>[2x]MQWSGARALEALLTVAGELRGP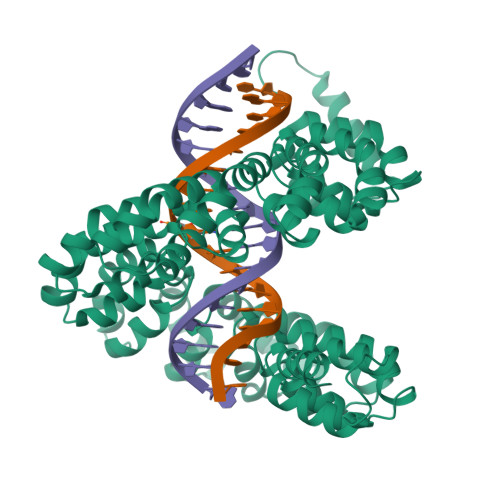PLQLDTGQLLKIAKRGGVTAVEAVHAWRNALTGAPLNLTPEQVVAIASHDGGKQALETVQRLLPVLCQAHGLTPQQVVAIASHDGGKQALETVQRLLPVLCQAHGLTPEQVVAIASHDGGKQALETVQALLPVLCQAHGLTPEQVVAIASNGGGKQALETVQRLLPVLCQAHGLTPQQVVAIASNGGGKQALETVQRLLPVLCQAHGLTPQQVVAIASHAGGKQALETVQRLLPVLCQAHGLTPQQVVAIASNNGGKQALETVQRLLPVLCQAHGLTPQQVVAIASHDGGKQALETVQRLLPVLCQAHGLTPQQVVAIASNNGGKQALETVQRLLPVLCQAHGLTPEQVVAIASNGGGKQALETVQRLLPVLCQAHGLTPEQVVAIASHDGGKQALETVQRLLPVLCQAHGLTPQQVVAIASNGGGRPALESIVAQLSRPDPALAALTNDHLVALACLGGRPALDAVKKLEHHHHHH(1S,2S)-2-phenyl-N-(pyridin-4-yl)cyclopropanecarboxamide | C15 H14 N2 O 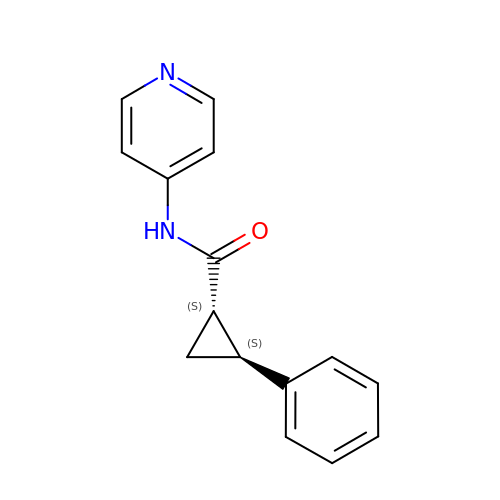| NOMFGVQIYPJHNJ-KGLIPLIRSA-N>[2x]EGFIDDSTLTGGIYYWQRERDRKDVTDGDKYKTNLSHSTWNANLDFQSGYAADMFGLDIAAFTAIEMAENGDSSHPNEIAFSKSNKAYDEDWSGDKSGISLYKAAAKFKYGPVWARAGYIQPTGQTLLAPHWSFMPGTYQGAEAGANFDYGDAG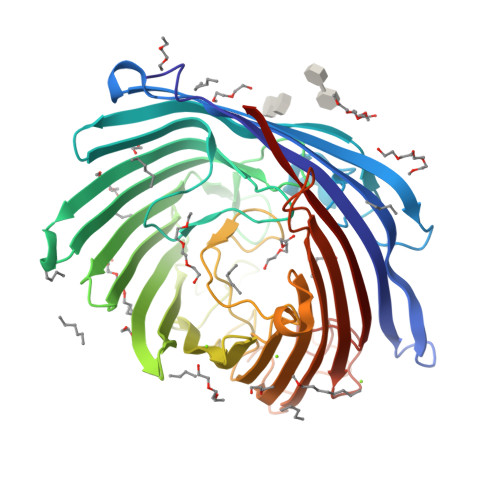ALSFSYMWTNEYKAPWHLEMDEFYQNDKTTKVDYLHSFGAKYDFKNNFVLEAAFGQAEGYIDQYFAKASYKFDIAGSPLTTSYQFYGTRDKVDDRSVNDLYDGTAWLQALTFGYRAADVVDLRLEGTWVKADGQQGYFLQRMTPTYASSNGRLDIWWDNRSDFNANGEKAVFFGAMYDLKNWNLPGFAIGASYVYAWDAKPATWQSNPDAYYDKNRTIEESAYSLDAVYTIQDGRAKGTMFKLHFTEYDNHSDIPSWGGGYGNIFQDERDVKFMVIAPFTIFHHHHHH> MATNFFIQPITEEAEAYYPPSVITNKRKDLGVDVYCCSDLVLQPGLNIVRLHIKVACEHMGKKCGFKIMARSSMCTHERLLILANGIGLIDPGYVGELMLKIINLGDTPVQIWAKECLVQLVAQGDHVPDHINILKRNQIFPLFAPTPRGEGRFGSTGEAG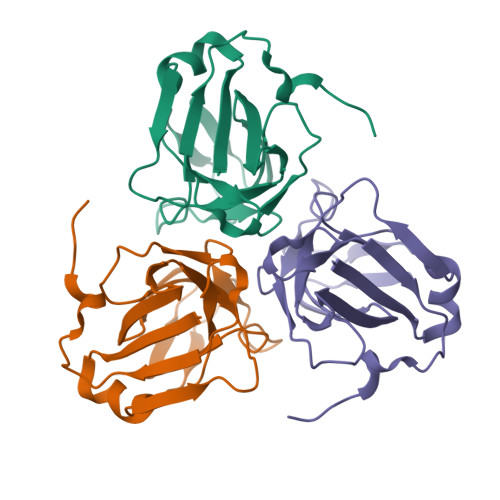IMRTHHHHHH>[4x]MAVPETRPNHTIYINNLNEKIKKDELKKSLHAIFSRFGQILDILVSR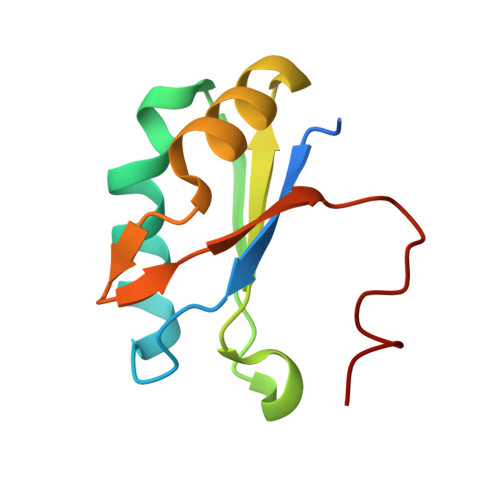SLKMRGQAFVIFKEVSSATNALRSMQGFPFYDKPMRIQYAKTDSDIIAKMW> KELGHEVLKPYDGWAAYGEGTTGGAMASPQNVFVVTNRTELIQALGGNNHTNQYNSVPKIIYVKGTIDLNVDDNNQPVGPDFYKDPHFDFEAYLREYDPATWGKKEVEGPLEEARVRSQKKQKDRIMVYVGSNTSIIGVGKDAKIKGGGFLIKNVDNVIIRNIEFEAPLDYFPEWDPTDGTLGEWNSEYDSISIEGSSHIWIDHNTFTDGDHPDRSLGTYFGRPFQQHDGALDIKNSSDFITISYNVFTNHDKVTLIGASDSRMADSGHLRVTLHHNYYKNVTQRLPRVRFGQVHIYNNYYEFSNLADYDFQYAWGVGVFSQIYA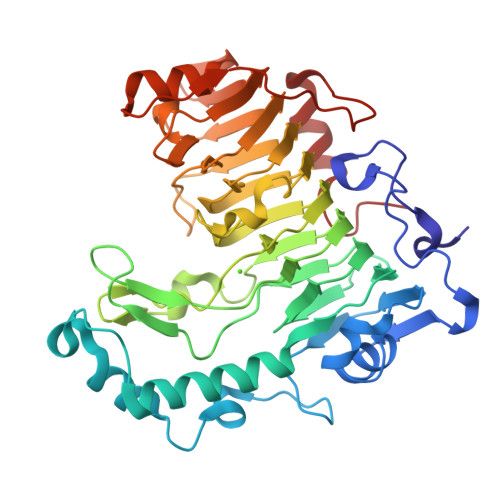QNNYFSFDWDIDPSLIIKVWSKNEESMYETGTIVDLPNGRRYIDLVASYNESNTLQLKKEVTWKPMFYHVIHPTPSVPALVKAKAGAGNLH>SNAAPQQINDIVHRTITPLIEQQKIPGMAVAVIYQGKPYYFTWGYADIAKKQPVTQQTLFELGSVSKTFTGVLGGDAIARGEIKLSDPTTKYWPELTAKQWNGITLLHLATYTAGGLPLQVPDEVKSSSDLLRFYQNWQPAWAPGTQRLYANSSIGLFGALAVKPSGLSFEQAMKTRVFQPLKLNHTWINVPSAEEKNYAWGYREGKAVHVSPGALDAEAYGVKSTIEDMARWVQSNLKPLDINEKTLQQGIQLAQSRYWQTGDMYQGLGWEMLDWPVNPDIIINGSDNKIALAARPVKPITPPTPAVRASWVHKTGATGGFG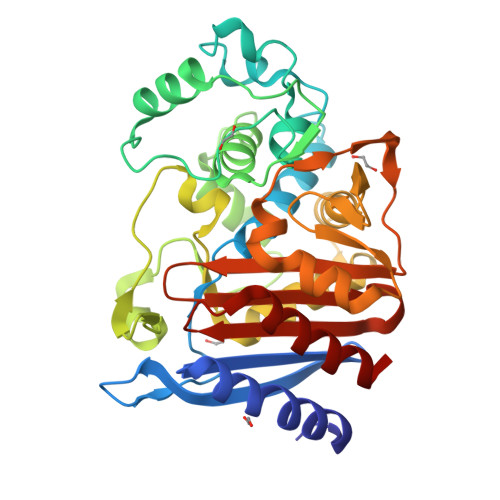SYVAFIPEKELGIVMLANKNYPNPARVAAAWQILNALQ[2x]>[4x]SGERVEDNELANYIAVIGLGGYYPGADSIDELWQNLANGVDCMSDFPADRWDHSKIYYKNRKVLGKTTCINGSFIKDVDKFDYSYFKMPKVYADHMSPEVRLFLQVAVHTFEDAGYSKETLLSRYNGDVGVLLGTMSNDYHYYGFESNVFRGSMASGSGMATIPMTVSYFYGLTGPSLFIDTMCSSSSTCIHTACQMLKHDETKMVLAGGLNLMYHPYTTVNTSQGNFTSITSESVNSYGVGADGTVIGEGIGAVLLKRLDRAIADRDQIYGVIKGSAMTNAGERNGFNVPNPDLQTLAIRQAMDQAKVHPSSISYIEGHGSGTKLGDPIEVLGLNNAFRWATDDKQFCYLGSIKSNIGHLLAASGIAGLTKTLLQFKHKQIAPSIHSSQLNQDIDFADTPFVVPQQLIEWRQPERIINGRKQVFPRRAGLTSIAAGGMNAHMIVEEYPEPADSAGQISEDQL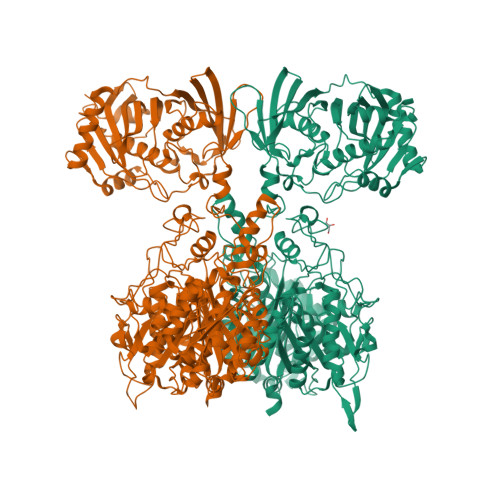VFVFSVHKLALLAQNLTSFRDWLASSEAPLAQIAYTLQVGKNNLRNRLAIRCRTRQALSRALNACIDGHYQSSADSKIFYRFQESDAVQPLESDLNDPLAPLLTQWLNGDSQVDWASLYAQPPVRISLPAYRFEKTRCWYTEEGYESSIVNPLMFKNKLHPLVAKNCSTPQPGAIFRTDFVEDELLDYVYSGRGGRRLSAFNFADVALAMPALASRFDGRTLSVSCAFEHYIADWTTVTGLEYRLFEIDSEQLELEFDFRRSGEQPTHLGFAVINPLTSDEPPLPQQWLDDARELLNRQALQAGRQLSAAEVSQRLAQAGYDFAPYLDHDGELTIGRSGLVLKGRPPVNRHNHYADNVQLSPYLATTIDKALYLLLDELGLPQGRVIVRNIERLCCYHTPAGGFSVVLSGIGLNDNELSLSLLVLDEREQICVKLDKVSLYLGKQEVASVDRKHSLLTGT>MTVSLRHTQVRDDVRLRLKMLEDIAQRMEAAVPGLRVELEGVEDKVNRFEKLPAEMAAG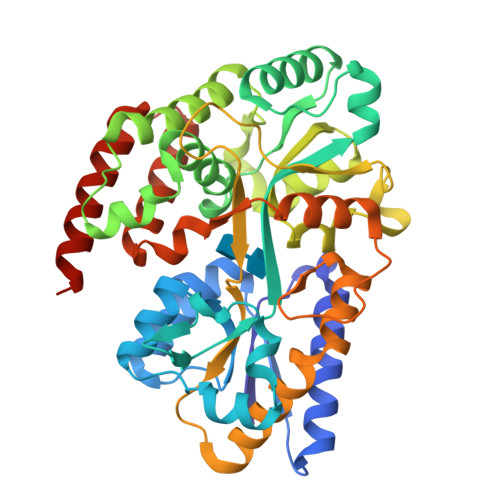NPPKIFDLFGGTDTAKYVKAGRLLELTPILNELGLKDKFPNLQEFTVDGKIYGLPTAYFVEGVFYNKQIFKQLNVDVPRRWEDLMDVAAKAKASGFVPFAFASSDGWVANMMLNTLWVRTAGDDSVPGFVRGTRRWTDPDVADGFKRYDTLLKKGYLQEGSLGQKYAEQQYAFREGRAAMMFDGSWASAALVDAGKTKIAEDIGFFSFPDVGGKGDGMINGGYSNGYGFSASLNEREKKAAVEFIKIMYSEEMQKRQLKESGILPAMKLSDLSGVHPVIREMIQASELRQFPAFDSIVQAKVRETLEMCMQELIGGRMTVEQVLDKMQKVQEDANRDMKKLEHHHHHH[2x]> MRERPHTSGHHGAGEARATAPSTVSPYGPEARAELSSRLTTLRNTLAPATNDPRYLQACGGEKLNRFRDIQCRRQTAVRADLNANYIQVGNTRTIACQYPLQSQLESHFRMLAENRTPVLAVLASSSEIANQRFGMPDYFRQSGTYGSITVESKMTQQVGLGDGIMADMYTLTIREAGQKTISVPVVHVGNWPDQTAVSSEVTKALASLVDQTAETKRNMYESKGSSAVADDSKLRPVIHCRAGVGRTAQLIGAMCMNDSRNSQLSVEDMVSQMRVQRNGIMVQKDEQLDVLIKLAEGQGRPLL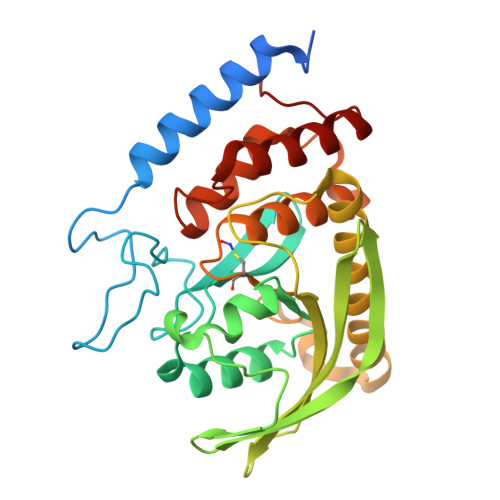NS>[4x]MGFLKGKKGLIVGVANNKSIAYGIAQSCFNQGATLAFTYLNESLEKRVRPIAQELNSPYVYELDVSKEEHFKS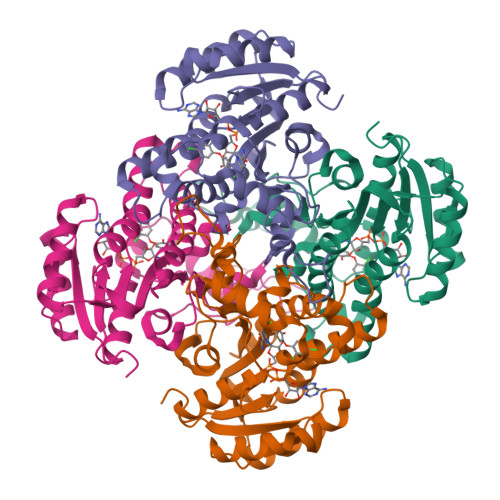LYNSVKKDLGSLDFIVHSVAFAPKEALEGSLLETSKSAFNTAMEISVYSLIELTNTLKPLLNNGASVLTLSYLGSTKYMAHYNVMGLAKAALESAVRYLAVDLGKHHIRVNALSAGPIRTLASSGIADFRMILKWNEINAPLRKNVSLEEVGNAGMYLLSSLSSGVSGEVHFVDAGYHVMGMGAVEEKDNKATLLWDLHKEQ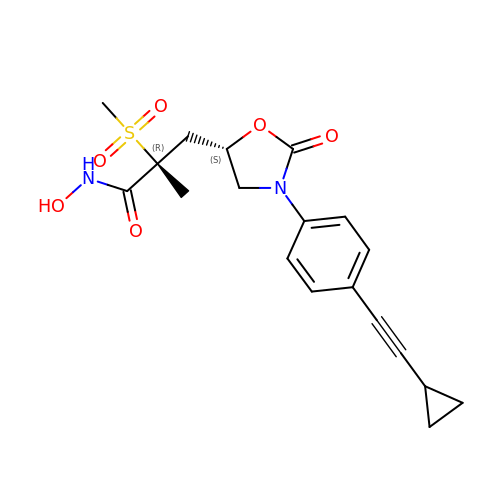(2R)-3-{(5S)-3-[4-(cyclopropylethynyl)phenyl]-2-oxo-1,3-oxazolidin-5-yl}-N-hydroxy-2-methyl-2-(methylsulfonyl)propanamide | C19 H22 N2 O6 S | ZXMGACHEILAVEA-QFBILLFUSA-N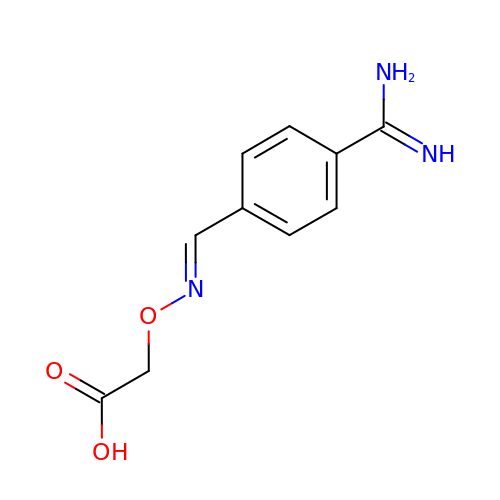(E)-2-(4-carbamimidoylbenzylideneaminooxy)acetic acid | C10 H11 N3 O3 | ZLBUXZJWFUDICQ-WLRTZDKTSA-N> SVIGRIHSFESCGTVDGPGIRFITFFQGCLMRCLYCHNRDTWDTHGGKEVTVEDLMKEVVTYRHFMNASGGGVTASGGEAILQAEFVRDWFRACKKEGIHTCLDTNGFVRRYDPVIDELLEVTDLVMLDLKQMNDEIHQNLVGVSNHRT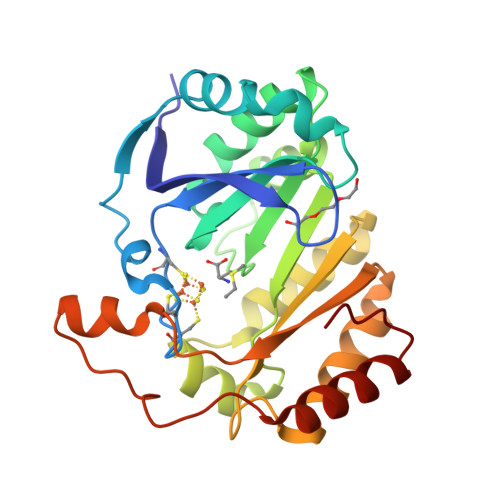LEFAKYLANKNVKVWIRYVVVPGWSDDDDSAHRLGEFTRDMGNVEKIELLPYHELGKHKWVAMGEEYKLDGVKPPKKETMERVKGILEQYGHKVMF> SGSFELRLKYFSNDHGRDNEGRCCSGESDGATGKCLGSCKTRFRVCLKHYQATIDTTSQCTYGDVITPILGENSVNLTDAQRFQNKGFTNPIQFPFSFSWPGTFSLIVEAWHDTNNSGNARTNKLLIQRLLVQQVLEVSS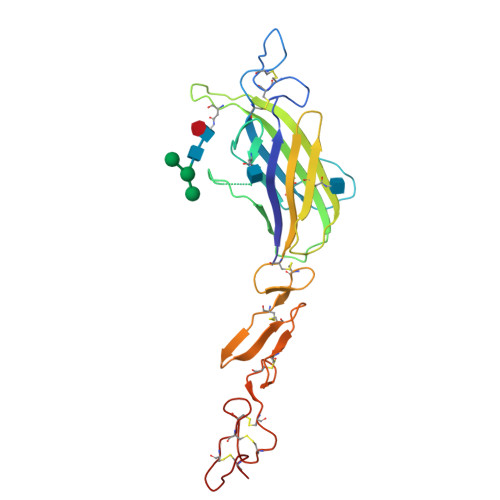EWKTNKSESQYTSLEYDFRVTCDLNYYGSGCAKFCRPRDDSFGHSTCSETGEIICLTGWQGDYCHIPKCAKGCEHGHCDKPNQCVCQLGWKGALCN(2S)-4-{4-[4-(benzyloxy)phenyl]-2-oxopyridin-1(2H)-yl}-N-hydroxy-2-methyl-2-(methylsulfonyl)butanamide | C24 H26 N2 O6 S | 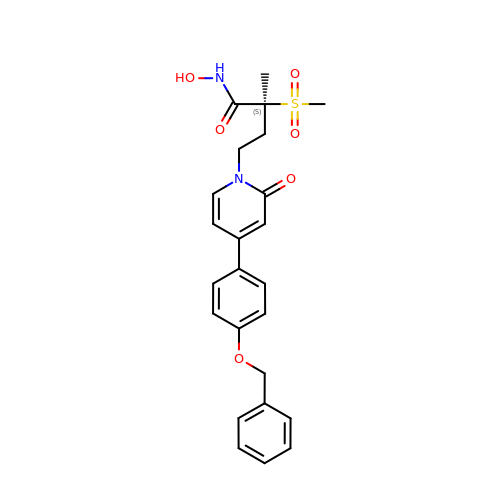QNBNKNVSGBGVPV-DEOSSOPVSA-N> MSLETKTPNDAKNQVQTHERMKTSSEHVTPL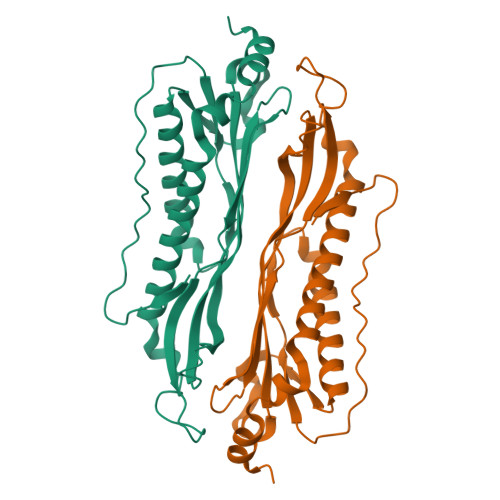DFNYPIHIVQAPQNHHVVGILTPRIQVSDNLKPYIDKFQDALINQIQTIFEKRGYQVLRFQDEKALNAQDKRKIFSVLDLKGWVGILEDLKMNLKDPNNPNLDTLVDQSSGSVWFNFYEPESNRVVHDFAVEVGTFQAMTYTYKHNNSGGLNSSNSIIHEYLEKNKEDAIHKILNRMYAVVMKKAVTELTKENIDKYREAIDRMKGFKSSMPQKKEGHHHHHH> QISVRGLAGVENVTELKKNFNRHLHFTLVKDRNVATPRDYYFALAHTVRDHLVGRWIRTQQHYYEKDPKRIYYLSLEFYMGRTLQNTMVNLALENACDEATYQLGLDMEELEEIEEDAGLGNGGLGRLAACFLDSMATLGLAAYGYGIRYEFGIFNQKICGGWQMEEADDWLRYGNPWEKARPEFTLPVHFYGRVEHTSQGAKWVDTQVVLAMPYDTPVPGYRNNVVNTMRLWSAKAPNDFNLKDFNVGGYIQAVLDRNLAENISRVLYPNDNFFEGKELRLKQEYFVVAATLQDIIRRFKSSKFGCRDPRVTNFDAFPDKVAIQLNDTHPSLAIPELMRVLVDLERLDWDKAWEVT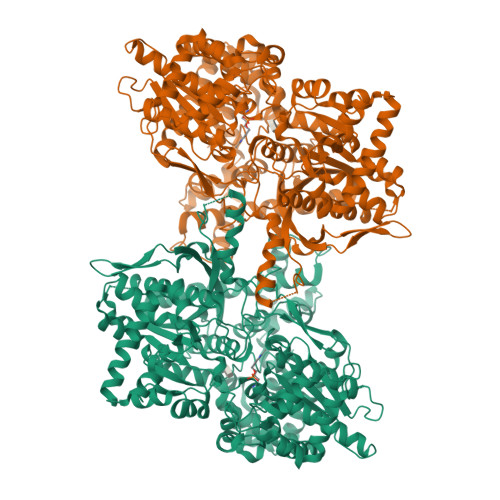VKTCAYTNHTVLPEALERWPVHLLETLLPRHLQIIYEINQRFLNRVAAAFPGDVDRLRRMSLVEEGAVKRINMAHLCIAGSHAVNGVARIHSEILKKTIFKDFYELEPHKFQNKTNGITPRRWLVLCNPGLAEIIAERIGEEYISDLDQLRKLLSYVDDEAFIRDVAKVKQENKLKFAAYLEREYKVHINPNSLFDVQVKRIHEYKRQLLNCLHVITLYNRIKKEPNKFVVPRTVMIGGKAAPGYHMAKMIIKLITAIGDVVNHDPVVGDRLRVIFLENYRVSLAEKVIPAADLSEQISTAGTEASGTGNMKFMLNGALTIGTMDGANVEMAEEAGEENFFIFGMRVEDVDRLDQRGYNAQEYYDRIPELRQIIEQLSSGFFSPKQPDLFKDIVNMLMHHDRFKVFADYEEYVKCQERVSALYKNPREWTRMVIRNIATSGKFSSDRTIAQYAREIWGVEPSRQRLPA>[2x]MRFIHALLLAGIAHSAYASEKLTFKTDLEKLEREKAAQIGVAIVDP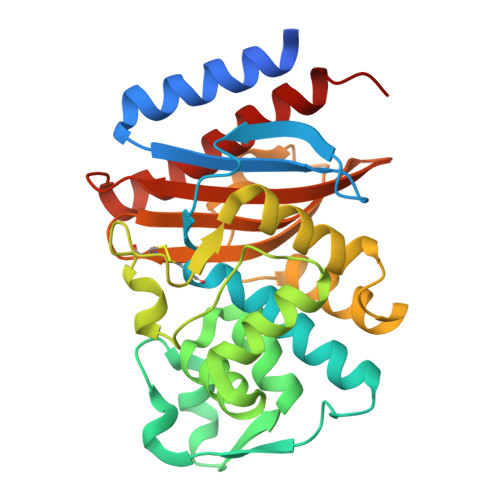QGEIVAGHRMAQRFAMCSTFKFPLAALIFERIDSGTERGDRKLSYGPDMIVEWSPATERFLASGHMTVLEAAQAAVQLSDNGATNLLLREIGGPAAMTQYFRKIGDSVSRLDRKEPEMSDNTPGDLRDTTTPIAMARTVAKVLYGGALTSTSTHTIERWLIGNQTGDATLRAGFPKDWVVGEKTGTCANGGRNDIGFFKAQERDYAVAVYTTAPKLSAVERDELVASVGQVITQLILSTDK Bacterial cytokinesis is initiated by the formation of a ring-like structure termed the Z-ring, a polymeric assembly of the essential tubulin homolog FtsZ at future division sites. Once formed, the Z-ring serves as a scaffold to recruit other cell division proteins that collectively constitute the divisome. FtsZ subunits have been suggested to interact through two putative sets of interfaces, longitudinal interfaces that join the subunits in a head-to-tail manner thereby forming a protofilament, and lateral interfaces that occur between protofilaments. However, unlike tubulin, which exhibits strong lateral interactions to form multi-stranded microtubules, FtsZ polymerizes into single-stranded protofilaments, and undergoes GTP hydrolysis-driven treadmilling.

To address the nature and in vivo role of FtsZ lateral interactions, we solved the structure of Mycobacterium tuberculosis FtsZ (MtbFtsZ) in a double-stranded protofilament state. We have now identified candidates for these interfaces in a new hexagonal crystal of MtbFtsZ, which has been determined to an Rfree factor of 27.3% at a resolution of 2.7 Å. Compared with our earlier MtbFtsZ structure, our newly determined MtbFtsZ structure is similarly double-stranded and reveals curved filaments in an antiparallel arrangement. However, in this new structure, the inter-protofilament interface is located at the external faces of helices H3, H4, and H5 in the N-terminal subdomain (lateral interface 2). By contrast, the lateral interface in the new MtbFtsZ structure is composed of basic residues Arg76, Lys77, Lys83, Arg119, and Lys120 and acidic residues Glu80, Glu87, and Glu153 from both interacting subunits, burying a larger surface area of ~870 Å2. These residues form charged complementary surfaces, suggesting the existence of electrostatic interactions. The charged residues involved in both lateral interfaces are generally conserved, indicating that they are functionally relevant. Comparison of this structure with that of MtbFtsZ in a different double-stranded protofilament state that we previously determined revealed two different inter-protofilament lateral interfaces. By contrast, when probing with the streptavidin conjugate, only single bands at both the monomer and the dimer positions (corresponding to the higher molecular weight band in the anti-FtsZ immunoblot) were detected. These photocrosslinking results clearly demonstrate that both lateral interfaces mediate interactions between FtsZ subunits in living cells. Mutagenesis of Lys121 revealed similar variability, with K121M and K121V able to complement. These results, together with those from double mutagenesis, suggest that lateral interactions are predominantly mediated by van der Waals interactions, which are sensitive to surface geometry; the charge complementarity may enhance these associations.

> MTPPHNYLAVIKVVGIGGGGVNAVNRMIEQGLKGVEFIAINTDAQALLMSDADVKLDVGRDSTRGLGAGADPEVGRKAAEDAKDEIEELLRGADMVLVTAGEGGGTGTGGAPVVASIARKLGALTVGVVTRPFSFEGKRRSNQAENGIAALRESCDTLIVIPNDRLLQMGDAAVSLMDAFRSADEVLLNGVQGITDLITTPGLINVDFADVKGIMSGAGTALMGIGSARGEGRSLKAAEIAINSPLLEASMEGAQGVLMSIAGGSDLGLFEINEAASLVQDAAHPDANIIFGTVIDDSLGDEVRVTVIAAGFDVSGPGRKPVMGETGGAHRIESAKAGKLTSTLFEPVDAVSVPLHTNGATLSIGGDDDDVDVPPFMRR>MKNVLVFLILLVALPALAQGHKPLEVIKIEDGVYLHTSFKNIEGYGLVDSNGLVVLDNNQAYIIDTPWSEEDTKLLLSWATDRGYQVMASISTHSHEDRTAGIKLLNSKSIPTYTSELTKKLLAREGKPVPTHYFKDDEFTLGNGLIELYYPGAGHTEDNIVAWLPKSKILFGGCLVRSHESEGLGYVGDASIS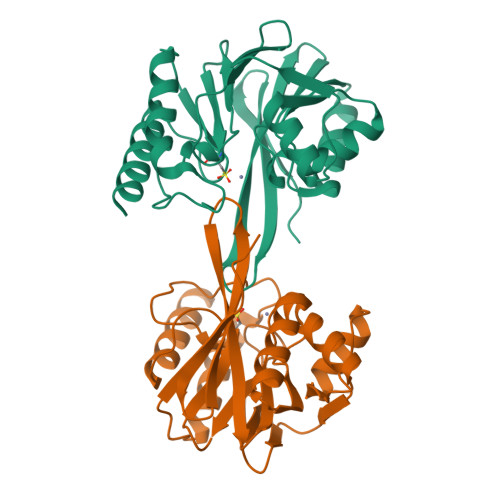SWADSIKNIVSKKYPIQMVVPGHGKVGSSDILDHTIDLAESASNKLMQPTAEASAD[2x]3-{[([1,1'-biphenyl]-3-yl)carbamoyl]amino}benzoic 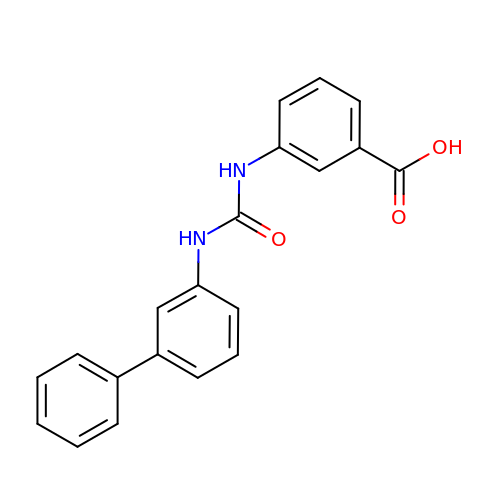acid | C20 H16 N2 O3 | FMMGJYWGPFRVFI-UHFFFAOYSA-N>GSSCDFVADVPPPKKGTDYDFYEAWGPVFEAEARFSKKTPIPSLGNMDSSKKEVEQFYAFWHRFDSWRTFEFLDEDVPDDSS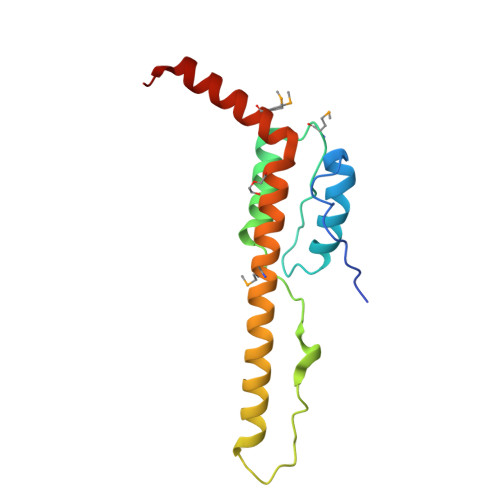NRDHKRYIERKNKAARDKKKTADMARLVKLVERAVSEDPRIKMFKEEEKKEKERRKWE[2x]>GMEVLDLVTGPDSVTEIEAFLNPRMGQPPTPESLTEGGQYYGWSRGINLATSDTEDSPGNNTLPTWSMAKLQLPMLNEDLTCDTLQMWEAVSVKTEVVGSGSLLDVHGFNKPTDTVNTKGISTPVEGSQYHVFAVGGEPLDLQGLVTDARTKYKEEGVVTIKTITKKDMVNKDQVLNPISKAKLDKDGMYPVEIWHPDPAKNENTRYFGNYTGG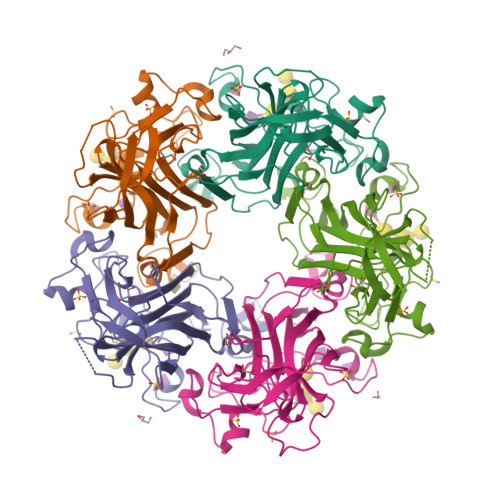TTTPPVLQFTNTLTTVLLDENGVGPLCKGEGLYLSCVDIMGWRVTRNYDVHHWRGLPRYFKITLRKRWVK[5x]> TENILRKSDEEIQKEITARVKALESMLIEQGILTTSMIDRMAEIYENEVGPHLGAKVVVKAWTDPEFKKRLLADGTEACKELGIGGLQGEDMMWVENTDEVHHVVVCTLCSCYPWPVLGLPPNWFKEPQYR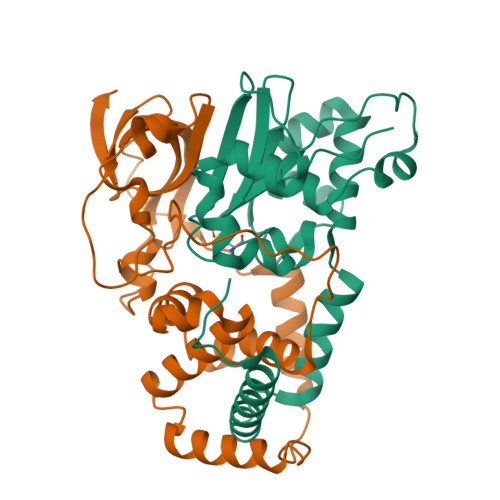SRVVREPRQLLKEEFGFEVPPSKEIKVWDSSSEMRFVVLPQRPAGTDGWSEEELATLVTRESMIGVEPAKAV;> MNGVYDVGGTDGLGPINRPADEPVFRAEWEKVAFAMFPATFRAGFMGLDEFRFGIEQMNPAEYLESPYYWHWIRTYIHHGVRTGKIDLEELERRTQYYRENPDAPLPEHEQKPELIEFVNQAVYGGLPASREVDRPPKFKEGDVVRFSTASPKGHARRARYVRGKTGTVVKHHGAYIYPDTAGNGLGECPEHLYTVRFTAQELWGPEGDPNSSVYYDCWEPYIELVDT NDM-1 has been reported to be a highly potent carbapenem-hydrolyzing, zinc-dependent MBL. NDM-1 is an extended spectrum zinc dependent β-lactamase capable of hydrolyzing nearly all classes of β-lactams, impairing the ability to treat life-threatening infections with intravenously and orally available carbapenems.. NDM-1 resembles the common β-lactamase fold, although it shows low sequence similarity to β-lactamases deposited in PDB (20–33% sequence identity). Our results show that NDM-1 is unique among other MBLs due to its enlarged and flexible active site, and explain the observed extended spectrum β-lactamase activity.

Three of our apoNDM-1 structures are zinc-free and are the first structures of a wild-type apo-enzyme in subclass B1. The model for NDM-1 Δ38 contains 226 residues (45–270) out of a possible 232 residues and 131 water molecules. The electron density maps obtained for the NDM-1 Δ38 structure allowed modeling of 226 residues of both A and B chains, except the 10 N-terminal residues including the three residues Ser-Asn-Ala left over from cloning, which are disordered and not included in the final model. The NDM-1 Δ38 models were refined against 2.0 Å data with a final Rwork of 19.5% and Rfree of 24.3%. In apoNDM-1 structure conformations of some of these residues are very similar to zinc-bound states (His120, Asp124, and His250), while others show somewhat different side chain orientations (His122, His189, and Cys208). Cys208 exists in two orientations in apo-state, one is similar to the zinc bound state and the other is rotated about 45 and 90 degrees in chain A and B, respectively. In the apoNDM-1 structure, two water molecules are coordinated by zinc-binding side chains, including Asp124, His122, and His250.

>[2x]SNAMETGDQRFGDLVFRQLAPNVWQHTSYLDMPGFGAVASNGLIVRDGGRVLVVDTAWTDDQTAQILNWIKQEINLPVALAVVTHAHQDKMGGMDALHAAGIATYANALSNQLAPQEGMVAAQHSLTFAANGWVEPATAPNFGPLKVFYPGPGHTSDNITVGIDGTDIAFGGCLIKDSKAKSLGNLGDADTEHYAASARAFGAAFPKASMIVMSHSAPDSRAAITHTARMADKLR>[2x]MAIGEFMVSLPRMVYPQPKVLTPCRKDVLVVTPWLAPIVWEGTFNIDILNEQFRLQNTTIGLTVFAIKKYVAFLKLFLETAEKHFMVGHRVHYYVFTDQPAAVPRVTLGTGRQLSVLEVRAYKRWQDVSMRRMEMISDFCERRFLSEVDYLVCVDVDMEFRDHVGVEILTPLFGTLHPGFYGSSREAFTYERRPQSQAYIPKDEGDFYYGGAFFGGSVQEVQRLTRACHQAMMVDQANGIEAVWHD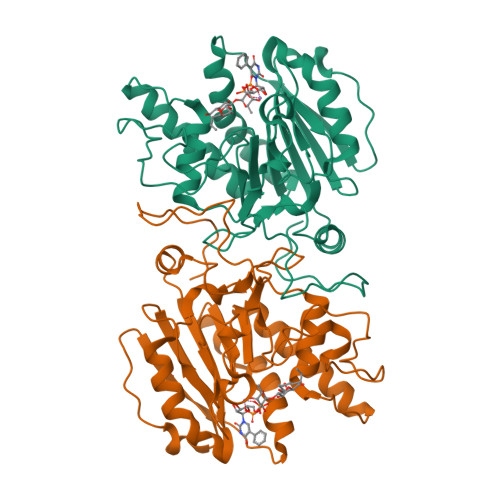ESHLNKYLLRHKPTKVLSPEYLWDQQLLGWPAVLRKLRFTAVPKNHQAVRNP>MHHHHHHSTPSIVIASAARTAVGSFNGAFANTPAHELGATVISAVLERAGVAAGEVNEVILGQVLPAGEGQNPARQAAMKAGVPQEATAWGMNQLCGSGLRAVALGMQQIATGDASIIVAGGMESMSMAPHCAHLRGGVKMGDFKMIDTMIKDGLTDAFYGYHMGTTAENVAKQWQLSRDEQDAFAVASYNKAEAAQKDGRFKDEIVPFIVKGRKGDITVDADEEIRGATLDSMAKLRPAFDKEGTVTAGNASGLNDGAAAALLMSEAEASRRGIQPLGRIVSWATVGVDPKVMGTGPIPASRKALERAGWKIGDLDLVEANEAFAAQACAVNKDLGWDPSIVNVNGGAIAIGH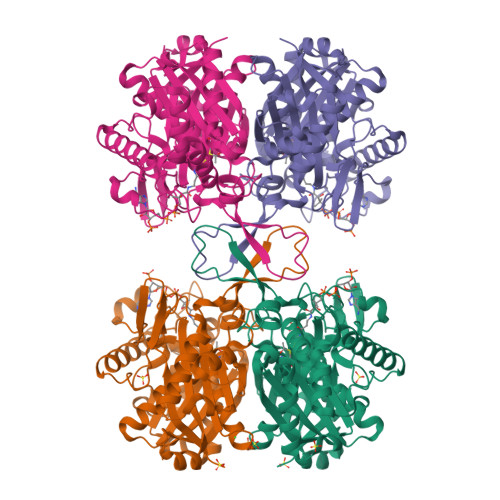PIGASGARILNTLLFEMKRRGARKGLATLCIGGGMGVAMCIESL[4x]>QYSSNTQQGRTSIVHLFEWRWVDIALECERYLAPKGFGGVQVSPPNENVAIHNPFRPWWERYQPVSYKLCTRSGNEDEFRNMVTRCNNVGVRIYVDAVINHMCGNAVSAGTSSTCGSYFNPGSRDFPAVPYSGWDFNDGKCKTGSGDIENYNDATQVRDCRLSGLLDLALGKDYVRSKIAEYMNHLIDIGVAGFRIDASKHMWPGDIKAILDKLHNLNSNWFPEGSKPFIYQEVIDLGGEPIKSSDYFGNGRVTEFKYGAKLGTVIRKWNGEKMSYLKNWGEG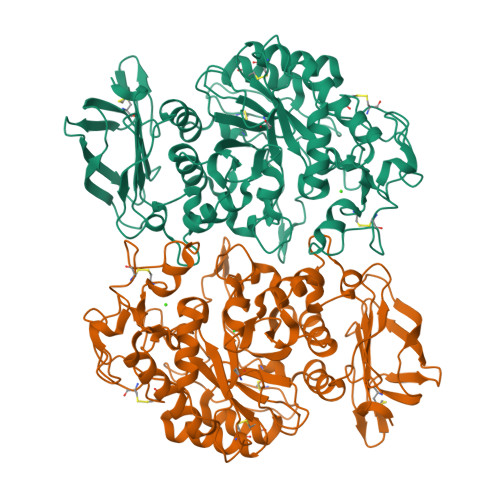WGFMPSDRALVFVDNHDNQRGHGAGGASILTFWDARLYKMAVGFMLAHPYGFTRVMSSYRWPRYFENGKDVNDWVGPPNDNGVTKEVTINPDTTCGNDWVCEHRWRQIRNMVNFRNVVDGQPFTNWYDNGSNQVAFGRGNRGFIVFNNDDWTFSLTLQTGLPAGTYCDVISGDKINGNCTGIKIYVSDDGKAHFSISNSAEDPFIAIHAESKL[2x]>MPKRTDIKSILILGAGPIVIGQACEFDYSGAQACKALREEGYRVILVNSNPATIMTDPEMADATYIEPIHWEVVRKIIEKERPDAVLPTMGGQTALNCALELERQGVLEEFGVTMIGATADAIDKAEDRRRFDVAMKKIGLETARSGIAHTMEEALAVAADVGFPCIIRPSFTMGG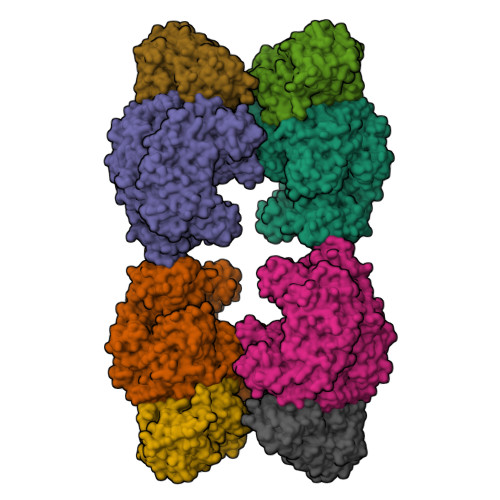SGGGIAYNREEFEEICARGLDLSPTKELLIDESLIGWKEYEMEVVRDKNDNCIIVCSIENFDAMGIHTGDSITVAPAQTLTDKEYQIMRNASMAVLREIGVETGGSNVQFAVNPKNGRLIVIEMNPRVSRSSALASKATGFPIAKVAAKLAVGYTLDELMNDITGGRTPASFEPSIDYVVTKIPRFNFEKFAGANDRLTTQMKSVGEVMAIGRTQQESLQKALRGLEVGATGFDPKVSLDDPEALTKIRRELKDAGADRIWYIADAFRAGLSVDGVFNLTNIDRWFLVQIEELVRLEEKVAEVGITGLNADFLRQLKRKGFADARLAKLAGVREAEIRKLRDQYDLHPVYKRVDTCAAEFATDTAYMYSTYEEECEANPSTDREKIMVLGGGPNRIGQGIEFDYCCVHASLALREDGYETIMVNCNPETVSTDYDTSDRLYFEPVTLEDVLEIVRIEKPKGVIVQYGGQTPLKLARALEAAGVPVIGTSPDAIDRAEDRERFQHAVERLKLKQPANATVTAIEMAVEKAKEIGYPLVVRPSYVLGGRAMEIVYDEADLRRYFQTAVSVSNDAPVLLDHFLDDAVEVDVDAICDGEMVLIGGIMEHIEQAGVHSGDSACSLPAYTLSQEIQDVMRQQVQKLAFELQVRGLMNVQFAVKNNEVYLIEVNPRAARTVPFVSKATGVPLAKVAARVMAGKSLAEQGVTKEVIPPYYSVKEVVLPFNKFPGVDPLLGPEMRSTGEVMGVGRTFAEAFAKAQLGSNSTMKKHGRALLSVREGDKERVVDLAAKLLKQGFELDATHGTAIVLGEAGINPRLVNKVHEGRPHIQDRIKNGEYTYIINTTSGRRAIEDSRVIRRSALQYKVHYDTTLNGGFATAMALNADATEKVISVQEMHAQIK[4x];>[4x]MIKSALLVLEDGTQFHGRAIGATGSAVGEVVFNTSMTGYQEILTDPSYSRQIVTLTYPHIGNVGTNDADEESSQVHAQGLVIRDLPLIASNFRNTEDLSSYLKRHNIVAIADIDTRKLTRLLREKGAQNGCIIAGDNPDAALALEKARAFPGLNGMDLAKEVTTAEAYSWTQGSWTLTGGLPEAKKEDELPFHVVAYDFGAKRNILRMLVDRGCRLTIVPAQTSAEDVLKMNPDGIFLSNGPGDPAPCDYAITAIQKFLETDIPVFGICLGHQLLALASGAKTVKMKFGHHGGNHPVKDVEKNVVMITAQNHGFAVDEATLPANLRVTHKSLFDGTLQGIHRTDKPAFSFQGHPEASPGPHDAAPLFDHFIELIEQYRKTAK>[2x]MIKKIGVLTSGGDAPGMNAAIRGVVRSALTEGLEVMGIYDGYLGLYEDRMVQLDRYSVSDMINRGGTFLGSARFPEFRDENIRAVAIENLKKRGIDALVVIGGDGSYMGAMRLTEMGFPCIGLPGTIDNDIKGTDYTIGFFTALSTVVEAIDRLRDTSSSHQ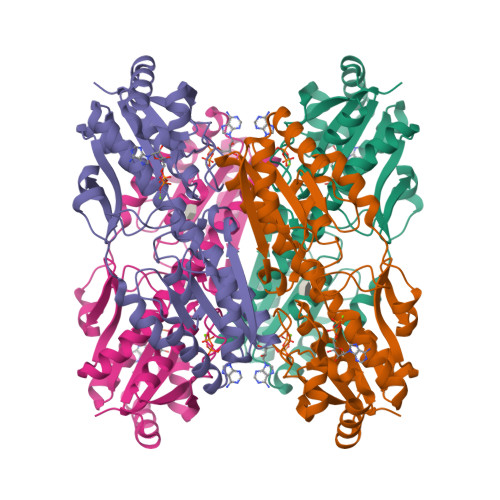RISVVEVMGRYCGDLTLAAAIAGGCEFVVVPEVEFSREDLVNEIKAGIAKGKKHAIVAITEHMCDVDELAHFIEKETGRETRATVLGHIQRGGSPVPYDRILASRMGAYAIDLLLAGYGGRCVGIQNEQLVHHDIIDAIENMKRPFKGDWLDCAKKLY6-CHLORO-N-[(3S)-1-(5-FLUORO-1,2,3,4-TETRAHYDROISOQUINOLIN-6-YL)-2-OXO-PYRROLIDIN-3-YL]NAPHTHALENE-2-SULFONAMIDE | C23 H21 Cl F N3 O3 S | 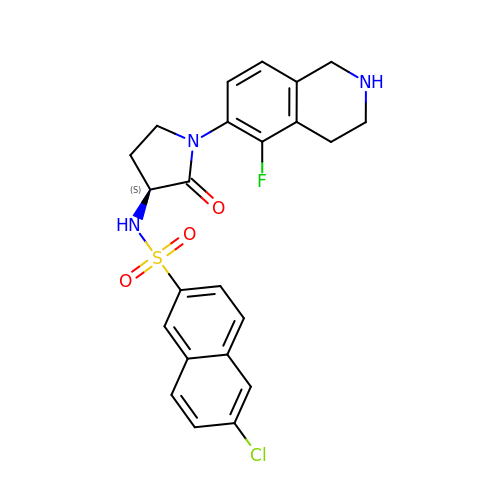BJOZEZZETKKCMQ-FQEVSTJZSA-N> AVPFY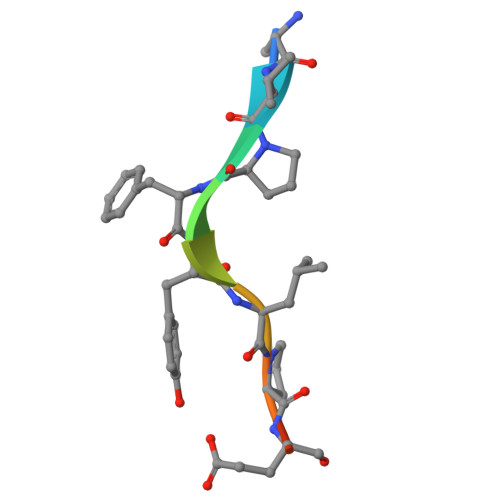LPEGG> MELKNSISDYTEAEFVQLLKEIEKENVAATDDVLYVLLEHFVKITEHPDGTDLIYYPSDNRDDSPEGIVKEIKEWRAA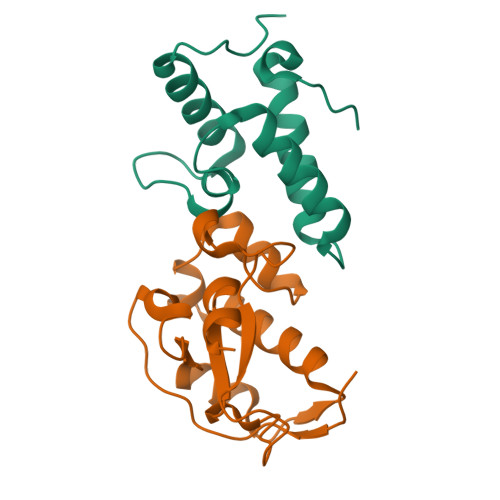NGKPGFKQG;> KRNKPGKATGKGKPVNNKWLNNAGKDLGSPVPDRIANKLRDKEFKSFDDFRKKFWEEVSKDPELSKQFSRNNNDRMKVGKAPQTRTQDVSGKRRSFELHHEKPISQNGGVYDMDNISVVTPKRAIDIH>MGSYLHEPPGDEPSMRIEQPKTADRAPEQVAIHICEPSKVVTESFPFSETAEPEAKSKNCPCPEIARIGPCPNKPPKIPINRGLSRISTNKSRPKSRFGEPSWPVESSLDLTSQSPVSPYREEAFSVENCGTAGSRRGSFARGTTSRAASSSRKDETKEGPDEKEVYQRVTAQLSARNQKRMTVKLMIELSVFLCLLGCLVCSLTVDGFKRYTVIGLDIWKWFLLLLVIFSGMLITHWIVHVAVFFVEWKFLMRKNVLYFTHGLKTSVEVFIWITVVLATWVMLIKPDVNQPHQTRKILEFVTWTIVTVLIGAFLWLVKTTLLKILASSFHLNRFFDRIQESVFHHSVLQTLAGRPVVELAQGISRTESQDGAGQVSFMEHTKTQNKKVVDVGKLHQMKQEKVPAWTMQLLVDVVSNSGLSTMSGMLDEDMVEGGVELDDDEITNEEQAIATAVRIFDNIVQDKVDQSYIDRVDLHRFLIWEEVDHLFPLFEVNEKGQISLKAFAKWVVKVYNDQAALKHALNDNKTAVKQLNKLVTAILIVMMIVIWLIVTGIATTKLIVLLSSQLVVAAFIFGNTCKTIFEAIIFVFVMHPFDVGDRCVIDGNKMLVEEMNILTTVFLKWDKEKVYYPNSILCTKAIGNFFRSPDQGDVLEFSVDFTTPVLKIGDLKDRIKMYLEQNLNFWHPQHNMVVKEIENVNKIKMALFVNHTINFQDFAEKNRRRSELVLELKKIFEELDIKYNLLPQEISIRNMGSGSLEVLFQ[7x]

Flycatcher1 (FLYC1), a MscS homolog, has recently been identified as a candidate mechanosensitive (MS) ion channel involved in Venus flytrap prey recognition. FLYC1 is an ortholog of prokaryotic MS ion channel MscS (mechanosensitive ion channel of small conductance), which functions as an osmotic release valve, and is perhaps the most extensively studied MS channel. FLYC1 comprises a homoheptamer with six TMs (TM1–TM6) per protomer and intracellular N and C termini. A glycine-containing hinge (G575) splits TM6 into two halves (TM6a and TM6b), and the β-rich C-termini of the FLYC1 protomers come together to form a hollow cytoplasmic cage.

A composite map was obtained from merging the C1 reconstruction and focused classification maps in a 6 up to 1 down protomer ratio, based on visible density from the C1 reconstruction. Topologically unique cytoplasmic flanking regions can adopt ‘up’ or ‘down’ conformations, making the channel asymmetric. Based on the composite ‘6 up 1 down’ model, we carried out additional MD simulations in the presence of negative membrane potentials of −450, −225, and −112.5 mV. The pore radius at the start is ~10% wider for the composite model at 3.1 Å radius, compared to the ‘all-up’ model. We also note that the pore constriction geometry across these three simulations is more well-preserved when the composite model was used. The wider pore constriction is accompanied by an increased number of chloride ion crossing events over the same simulation timescale, with a conductance estimation much closer to the electrophysiological measurements of the stretch-activated currents. Our MD simulations support the idea of passage of chloride in an ‘all-up’ state at −425 mV and a ‘6 up 1 down’ state at −450 mV, with the latter exhibiting an estimated conductance closer to electrophysiology measurements. Our observation that the channel adopts asymmetric assemblies with protomers adopting either up or down states is likely to add further complexity to the FLYC1 gating mechanism.>[2x]MIFPKQYPIINFTTAGATVQSYTNFIR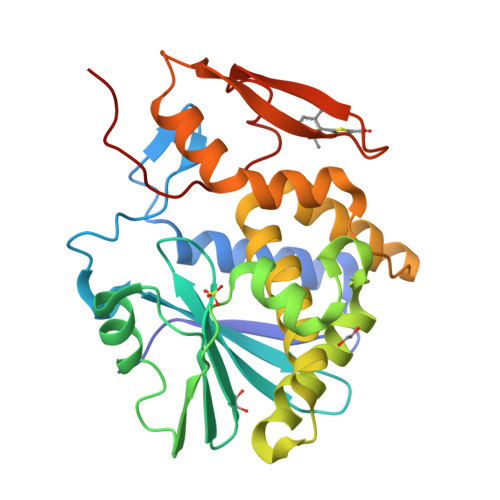AVRGRLTTGADVRHEIPVLPNRVGLPINQRFILVELSNHAELSVTLALDVTNAYVVGYRAGNSAYFFHPDNQEDAEAITHLFTDVQNRYTFAFGGNYDRLEQLAGNLRENIELGNGPLEEAISALYYYSTGGTQLPTLARSFIICIQMISEAARFQYIEGEMRTRIRYNRRSAPDPSVITLENSWGRLSTAIQESNQGAFASPIQLQRRNGSKFSVYDVSILIPIIALMVYRCAPPPSSQF> SCKNTDSRCKARQLELNERTCR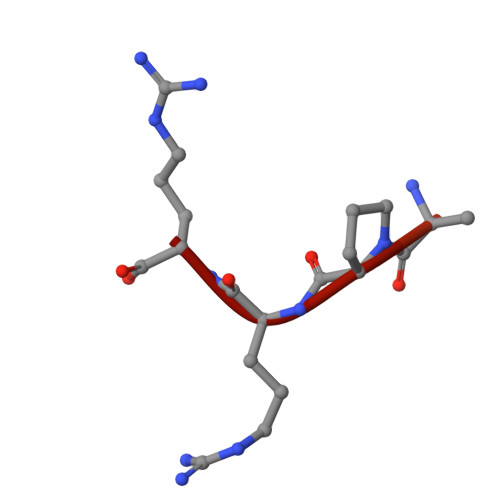CDKPRR>[2x]MEHICGTSRIAGFRFSLYPMTDDFISVIKS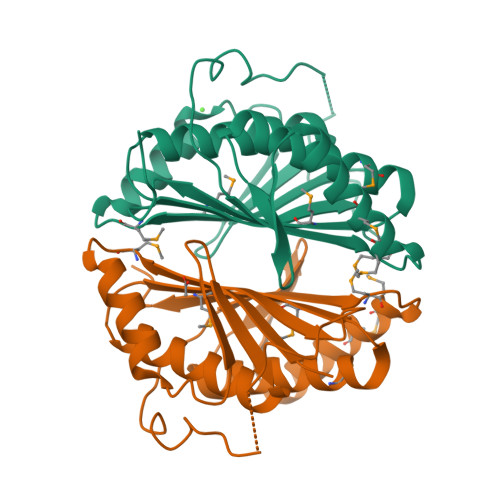ALAATDTSKVWTKTDHISTVLRGSIDHVFDAAKAIYLHAANSEQHIVMNGTFSIGCPGDTQGDTYLSKGDKRVNEDAVRGLKAEAPCQFALYPMNEPDYMGLIMEAVDIAKAQGTFVQGVHYASELDGDAHDVFSTLEAVFRMAEQQTNHITMTVNLSANSPSRKNRKQG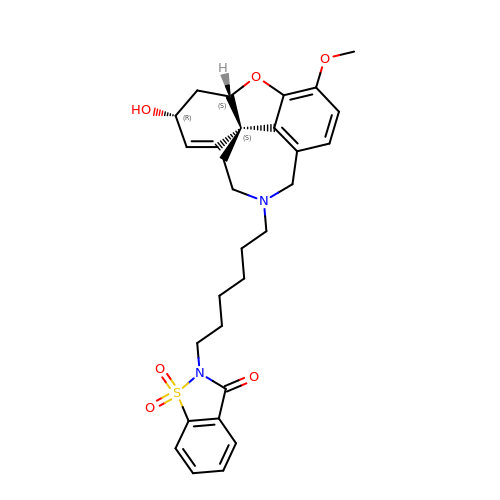2-{6-[(4aS,6R,8aS)-6-hydroxy-3-methoxy-5,6,9,10-tetrahydro-4aH-[1]benzofuro[3a,3,2-ef][2]benzazepin-11(12H)-yl]hexyl}-1,2-benzisothiazol-3(2H)-one 1,1-dioxide | C29 H34 N2 O6 S | VAEMEXGGRSPJEF-LOMAHXHCSA-N>[2x]DVTNAEKLVYKYTNIAHSANPMYEAPSITDGKIFFNRKFKTPSGKEAACASCHTNNPANVGKNI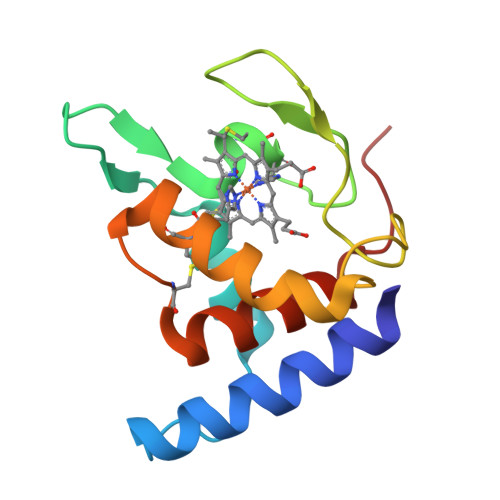VTGKEIPPLAPRVNTKRFTDIDKVEDEFTKHCNDILGADCSPSEKANFIAYLLTETKPTK Bacteriophage T5, a representative member of the T5-like family of siphophages, serves as an excellent model for studying the assembly, infection, cell wall perforation, and DNA ejection mechanisms of this phage family. In this study, we used cryo-electron microscopy (cryo-EM) to determine the structures of mature T5 (a laboratory-adapted, fiberless T5 mutant) and urea-treated empty T5 (lacking the tip complex) at near-atomic resolutions. The T5 head comprises 775 copies of MCP gp8, arranged into 11 pentons and 120 hexons, forming an icosahedral shell with a triangle number (T) of 13. The T5 tail, which comprises 40 trimeric rings of the TTP and a distal tip complex, is connected to a unique five-fold vertex of the head by the connector complex.

We obtained a high-resolution head map of mature T5 at a resolution of 3.9 Å by using icosahedral reconstruction. Using the local reconstruction method, we further improved the three-fold region of the head to a resolution of 3.4 Å. In comparison with the previous study of the T5 head, we built a more accurate atomic model of the pb8 monomer from residues 164–457 (out of 458 residues) based on our high-resolution density map. MCP pb8 adopts a canonical HK97-like fold and can be divided into four domains: an extended N-arm (residues 164–191), a P-domain (residues 192–205, 245–306, and 407–451), an E-loop domain (residues 206–244), and a complex A-domain (residues 307–406, and 452–457). During the maturation of the capsid, the first 160 residues of the N-terminus of pb8 undergo proteolytic cleavage, and this process also occurs in the MCPs of E217 and HK97. The asymmetric unit of the icosahedral head comprises 13 MCP gp8 monomers (a fifth penton, a hexon I, and a hexon II) and 2 pb10 monomers. The center of each hexon is adorned with a decorating protein pb10, which comprises an α-helical domain and an immunoglobulin (Ig)-like domain. We resolved only the α-helical domain, from residues 2 to 68 (out of 164 residues), which contains five α-helices: α1 (residues 4–10), α2 (residues 17–24), α3 (residues 25–30), α4 (residues 33–41), and α5 (residues 49–62). A structural comparison of our α-helical domain with the nuclear magnetic resonance (NMR) structure of pb10 in solution reveals that the α1 and α2 of the pb10 monomer undergo substantial conformational changes from the solution state to the assembled state. In contrast, our high-resolution structure indicated that the binding sites of pb10 were consistent in all hexons, likely due to minor conformational changes in the centers of the two types of hexons.

>MTIDINKLKEELGLGDLAKSLEGLTAAQKAQEAERMRKEQEEKELARMNDLVSKAVGEDRKRLEEALELVKSLDEKSKKSNELFAQTVEKQQETIVGLQDEIKSLLTAREGRSFVGDSVAKALYGTQENFEDEVEKLVLLSYVMEKGVFETEHGQRHLKAVNQSSSVEVSSESYETIFSQRIIRDLQKELVVGALFEELPMSSKILTMLVEPDAGKATWVAASTYGTDTTTGEEVKGALKEIHFSTYKLAAKSFITDETEEDAIFSLLPLLRKRLIEAHAVSIEEAFMTGDGSGKPKGLLTLASEDSAKVVTEAKADGSVLVTAKTISKLRRKLGRHGLKLSKLVLIVSMDAYYDLLEDEEWQDVAQVGNDSVKLQGQVGRIYGLPVVVSEYFPAKANSAEFAVIVYKDNFVMPRQRAVTVERERQAGKQRDAYYVTQRVNLQRYFANGVVSGTYAAS[12x];>[2x]MIDYSGLRTIFGEKLPESHIFFATVAAHKYVPSYAFLRRELGLSSAHTNRKVWKKFVEAYGKAIPPAPPAPPLTLSKDLTASMSVEEGAALTLSVTATGGTGPYTYAWTKDGSPIPDASGATYTKPTAAAEDAGSYKVTVTDSKQVSKDSTTCAVTVNPTVPGG>[2x]MGHHHHHHEFMAKR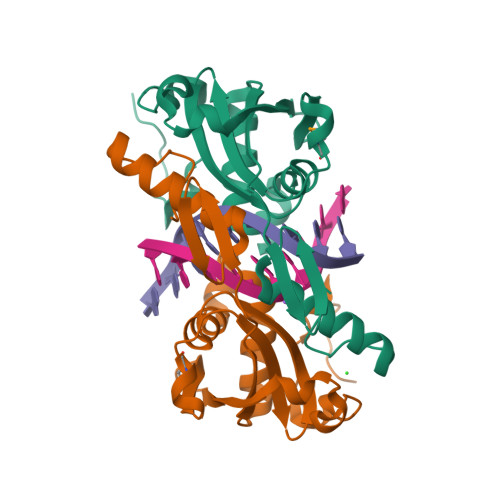KSDIILKSVDDLKDEIDYKDFEYKEYFNLLCELVPNNSLEKLEINAIDEKNMKNEGLVYVFVIQGKIFKIGHSITPITKRVQSYNCGKVEYRKNGTCSTTNYFVLQSLLKINKIVQVYAFFPEQPTYTLFGKTYQDSFSTSKRAENVILENFIKNHNKKPIGCTQT> AYTFDSTMLDTNSGESIDVSLFNQGLQLPGNYFVNVFVNGRKVDSGNIDFRLEKHNGKELLWPCLSSLQLTKYGIDIDKYPDLIKSGTEQCVDLLAIPHSDVQFYFNQQKLSLIVPPQALLPRFDGIMPMQLWDDG;> ADLTASTTATATLVEPARITLTYKEGAPITIMDNGNIDTELLVGTLTLGGYKTGTTSTSVNFTDAAGDPMYLTFTSQDGNNHQFTTKVIGKDSRDFDISPKVNGENLVGDDVVLATGSQDFFVRSIGSKGGKLAAGKYTDAVTVTVSNQ;> AQPDIKFASKEYGVTIGESRIIYPLDAAGVMVSVKNTQDYPVLIQSRIYDENKEKESEDPFVVTPPLFRLDAKQ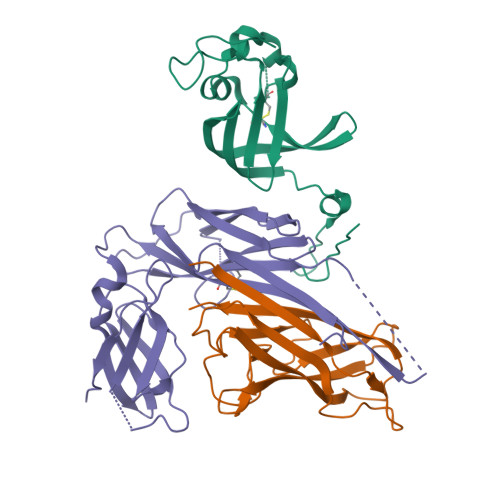QNSLRIAQAGGVFPRDKESLKWLCVKGIPPKDEDIWVDDATNKQKFNPDKDVGVFVQFAINNCIKLLVRPNELKGTPIQFAENLSWKVDGGKLIAENPSPFYMNIGELTFGGKSIPSHYIPPKSTWAFDLPKGLAGARNVSWRIINDQGGLDRLYSKNVTL>[2x]HHHHHHSSGLEVLFQGTTHRHLTREEEPQTPDEASLDLAATDGIRLGDRLRGLWDLRLVGGDAELPGLPREGLQLVLDVAPKGRGLIGYLDTPERLLAAEPPRFRVLGDLLGASSASIRWRLVDQASGSVAPTHDCSAVFDEVWADYANAGDGTLSGRIQRLERSPLSPNEDFRFVAVKRHFPLAHERIVLNEKLLGWLVSPQHRLFHQLWHASRDKWHRLSEKQRNALRGVGWQPGPLDRERDARGPRKDRNASGIDFFFMHRHMLHTARSMQDLPSWERLPRPVVPLEYDRPGFIRYFDNPDGFSVPPAWVAVDDDEYSEWLHGLKSAEAYHANFLVWESQYQDPAYLAKLTLGQFGSELELGMHDWLHMRWASVTRDPSNGAPVMTDRFPADFAPRWFRPENDF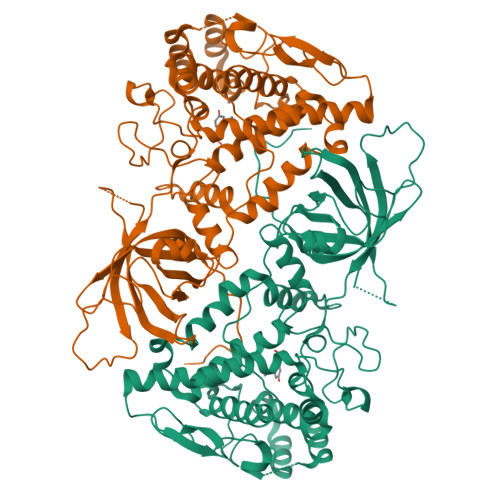LGDPFSSHVNPVFWSFHGWIDDRIEDWYRAHERFHPGEVQRREVEGIQWFAPGRWVEVGDPWLGPATHGCGLSDVQASSNSVELDVETMKLALRIIFSEEDQLSGWLKRAPRRPWYARNLKLARDQLRR Members of the myomesin protein family function as molecular bridges that connect major filament systems in the central M-band of muscle sarcomeres, which is a central locus of passive stress sensing. To unravel the mechanism of molecular elasticity in such filament-connecting proteins, we have determined the overall architecture of the complete C-terminal immunoglobulin domain array of myomesin by X-ray crystallography, electron microscopy, solution X-ray scattering, and atomic force microscopy. Our data reveal a dimeric tail-to-tail filament structure of about 360 Å in length, which is folded into an irregular superhelical coil arrangement of almost identical α-helix/domain modules. The myomesin filament can be stretched to about 2.5-fold its original length by reversible unfolding of these linkers, a mechanism that to our knowledge has not been observed previously.

First, we determined the overall architecture of the complete myomesin domain array, including Ig domains My9–My10–My11–My12–My13, from crystal structures of a total of three filament fragments: the My9–My11 triplet, determined at 2.5 Å resolution; the My10–My11 doublet, at 1.9 Å resolution; and the homodimeric My11–My13 triplet at 3.5 Å resolution. As the available independent structures of helix-connected Ig domain doublets show only limited variation in terms of domain/domain arrangements, a reliable overall structural model of the complete C-terminal myomesin Ig domain array My9–My13 can be generated. This reveals a tail-to-tail filament structure with an overall length of 360 Å and a pronounced zigzag-type arrangement within the central, C-terminal myomesin dimerization module (My13), followed by a superhelical coil arrangement towards the two symmetrical distal ends. The right-handed superhelix is defined by almost constant twist angles of neighboring My domains of 26–27°, except the arrangement of My12–My13, which has an average twist angle of 68° and thus appears to be less regular than preceding parts My9–My10–My11–My12 of the filament. Whereas long six-turn helices are found in the My10–My11 and My12–My13 connecting segments, the corresponding helices in the other two connecting segments, My9–My10 and My11–My12, are slightly shorter, with about four turns each. Because of the smaller length of their linkers, My9–My10 and My11–My12 show limited direct interactions in their respective Ig doublets, whereas in the other two doublets, My10–My11 and My12–My13, the neighboring My domains are too far away from each other to form an interface. The complete filament structure of the My9–My13 dimer therefore is defined by an arrangement of nine rigid bodies, comprising eight Ig domains and the central My13 dimer. Although the precise orientation of different filament parts of myomesin in the sarcomere is unknown, available experimental data lead to a model in which the dimeric link via the C-terminal My13 domain in myomesin filaments is across the central M-line.

>GIDPFTGPHFVEYLSWEVTGECNVLLKCKVANIKKETHIVWYKDEREISVDEKHDFKDGICTLLITEFSKKDAGIYEVILKDDRGKDKSRLKLVDEAFKELMMEVCKKIALSATDLKIQSTAEGIQLYSFVTYYVEDLKVNWSHNGSAIRYSDRVKTGVTGEQIWLQINEPTPNDKGKYVMELFDGKTGHQKTVDLSGQAYDEAYAEFQRLKQAAIAEKNRARVLGGLPDVVTIQEGKALNLTCNVWGDPPPEVSWLKNEKALASDDHCNLKFEAGRTAYFTINGVSTADSGKYGLVVKNKYGSETSDFTVSVFIPE[4x]SecA is an evolutionarily conserved and essential ATPase that is required for protein translocation in bacteria. The catalytic core of SecA (amino acids ~1–832 in E. coli) contains five domains: nucleotide binding domain-1 (NBD1; amino acids 9–220 and 378–411), the polypeptide crosslinking domain (PPXD; 221–377), nucleotide binding domain-2 (NBD2; 412–620), the α-helical scaffold domain (HSD; 621–672 and 756–832) and the α-helical wing domain (HWD; 673–755). In addition to the catalytic core, most SecA proteins contain a relatively long C-terminal tail (CTT; also known as the C-terminal linker [Hunt et al., 2002]), whose function is not well understood. In E. coli, the CTT (833-901) contains of a small metal binding domain (MBD; 878–901) and a structurally flexible linker domain (FLD; 833–877).

SecAΔMBD crystallised as a symmetric dimer in a head-to-tail configuration. Consistent with previous studies, the structure of the PPXD was less well defined relative to the other domains of the catalytic core, consistent with the idea that the PPXD is structurally mobile. However, because the FLD was not resolved, its effect on the structure of SecA could not be determined. To investigate how the CTT affects the conformation of SecA in solution, we investigated the structures of SecA, SecAΔCTT and SecAΔMBD using small-angle x-ray scattering (SAXS). The resulting models suggested that the PPXD was positioned considerably closer to NBD2 (i.e. more ‘open’) in SecA and SecAΔMBD than in SecAΔCTT (p=2.0×10−5 and 1.1 × 10−7, respectively). In models of SecAΔMBD and SecAΔCTT, the PPXDs in the two protomers of the dimers were positioned asymmetrically (p=1.8×10−8 and 0.0085, respectively). Disruption of the MBD alone (i) increases the affinity of SecA for the ribosome, (ii) decreases the affinity of SecA for substrate protein, (iii) inhibits the ATPase activity of SecA, (iv) increases the thermal stability of SecA, (v) prevents SecA from undergoing a conformational change upon binding to nascent substrate protein and (vi) causes a defect in SecA function in vivo. However, disruption of both the MBD and the FLD results in a protein that behaves very similarly to full-length SecA, indicating that the FLD mediates these effects. Our work suggests that enclosure of the FLD by the PPXD has the opposite effect—that is, autoinhibition of SecA. We propose that the MBD is the key for unlocking this autoinhibited conformation in the full-length protein.

> RNDRTLRRMRKVVNIINAMEPEMEKLSDEELKGKTAEFRARLEKGEVLENLIPEAFAVVREASKRVFGMRHFDVQLLGGMVLNERCIAEMRTGEGKTLTATLPAYLNALTGKGVHVVTVNDYLAQRDAENNRPLFEFLGLTVGINLPGMPAPAKREAYAADITYGTNNEYGFDYLRDNMAFSPEERVQRKLHYALVDEVDSILIDEARTPLIISGPAEDSSEMYKRVNKIIPHLIRQEKEDSETFQGEGHFSVDEKSRQVNLTERGLVLIEELLVKEGIMDEGESLYSPANIMLMHHVTAALRAHALFTRDVDYIVKDGEVIIVDEHTGRTMQGRRWSDGLHQAVEAKEGVQIQNENQTLASITFQNYFRLYEKLAGMTGTADTEAFEFSSIYKLDTVVVPTNRPMIRKDLPDLVYMTEAEKIQAIIEDIKERTAKGQPVLVGTISIEKSELVSNELTKAGIKHNVLNAKFHANEAAIVAQAGYPAAVTIATNMAGRGTDIVLGGSWQAEVAALENPTAEQIEKIKADWQVRHDAVLEAGGLHIIGTERHESRRIDNQLRGRSGRQGDAGSSRFYLSMEDALMRIFASDRVSGMMRKLGMKPGEAIEHPWVTKAIANAQRKVESRNFDIRKQLLEYDDVANDQRRAIYSQRNELLDVSDVSETINSIREDVFKATIDAYIPPQSLEEMWDIPGLQERLKNDFDLDLPIAEWLDKEPELHEETLRERILAQSIEVYQRKEEVVGAEMMRHFEKGVMLQTLDSLWKEHLAAMDYLRQGIHLRGYAQKDPKQEYKRESFSMFAAMLESLKYEVISTLSKVQVRMP>[2x]DEPNQPSTPEAVTKTVTIDASKYETWQYFSFSKGEVVNVTDYKNDLNWDMALHRYDVRLNCGES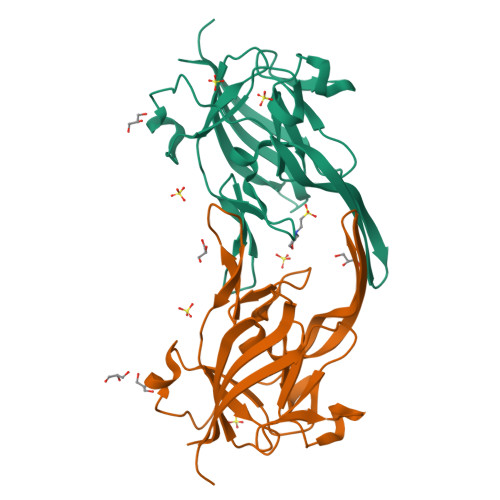GKGKGGAVFSGKTEMDQATTVPTDGYTVDVLGRITVKYEMGPDGHQMEYEEQGFSEVITGKKNAQGFASGGWLEFSHGPAGPTYKLSKRVFFVRGADGNIAKVQFTDYQDAELKKGVITFTYTYPVK> MAGERFPADFVWGAATAAYQIEGAVREDGRGVSIWDTFSHTPGKIADGTTGDVACDSYHRYGEDIGLLNALGMNAYRFSIAWPRIVPLGAGPINQAGLDHYSRMVDALLGAGLQPFVTLYHWDLPQPLEDRLGWGSRATATVFAEYADIVVRQLGDRVTHWATLNEPWCSAMLGYYLGVHAPGHTDLKRGLEASHNLLLGHGLAVQAMRAAAPQPLQIGIVLNLTPTYPASDS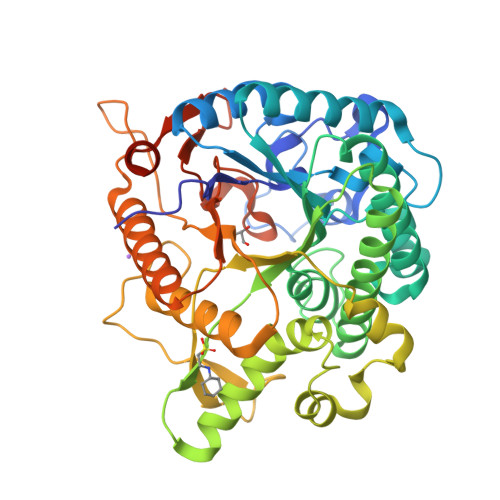PEDVAAARRFDGFVNRWFLDPLAGRGYPQDMLDYYGAAAPQANPEDLTQIAAPLDWLGVNYYERMRAVDAPDASLPQAQRLDDPDLPHTADREVYPEGLYDILLRLHNDYPFRPLYITENGCALHDEIAEDGGIHDGQRQAFFEAHLAQLQRALAAGVPLKGYFAWSLLDNFEWAMGLSMRYGICYTNFETLERRIKDSGYWLRDFIAGQRGKLAALEHHHHHH> KYSKRIAWMKTTICDSLQLKDMIVEESFQYEKNKNLLEQFLSGEGLNKIFAYYQVQEQAQNDDIKDTGAQDPVLFFTTGDLEKIQDKAVWFLRITNPADDKKKASQQDGNDNDIIFGEITPNTVPMLNALMESVYSRQIDHIITEKIQFWGVAEEEQVLEFQQHSNKFSSEVREAINLMSPGTEHFKLDYEAISGLSESEKMQHYEMKFNEWINLISSQLNDDSEVRKDEKDAGPATELIYWRSRMQKITNWSEQLKSKDFQIVKASLQRHKNHDNQRPRGDESLSKLMMEYNRLDLLLTDKLNEAKDNVKYLTTLEKFIEPLYNGTPQQIIDTLPALMNAIKMIHTIARFYNTTDKMTGLFIKITNQMIKNCKDRILNKKDNGDNPSLYKMIWEQDPAELIEVLGSCIKLYCEYKKCYNDTKEKVADMPKGKTFDFSDAQIFGKFDTFVRRLQKLIEIFSNIQQFNALAKHNLEGMDVLTNKFKKIIDDFKKKGHNLLDTANNKFDRDWVEFNVEISHLDGELQNFIDNNFNRFRNIEYSLKLLHKFQSTIKRDSLKHNLTSRYNAILHNYATELDTIQRVFQDQKSNPPLVRNMPPEAGKIIWARHLFQKITGPINIFPENVINSTEIRRYYGSYNTLGKQLTIYEMWFYQDWVNKIEQSKAALQATLIVRHDENKKLYVNFDLEIMQLIREAKCLDRQGIEIPESARIILLQEDKFKTYYNELLYALKEYERINSKIKPICKNLLLPHIEDLDLKLRPGMVTLTWTSMNIESYLYYVHQGLKKLEQLIINVNDIIENRIENNLKTVSKVVLVHLPQDTKPLSLDSFVQLQEEYINSKTDFLTSKNVEVERAVDDLLQTIMLYPLDPHVDPVLPEETKRIKRYYFWYFYQALLNSTQNSLNAMKYRVCGKKIPGANTLQNLKPFFQVEVQLNGDKVTLNPSLQEIQKSINRAATAVLRCSKHLYNWDQQNKDSTDKATFYDMIACDKEIVKVILLLTGSIQGTKNKVNEFLSGFTKFEWLCKESIQESIKKFSKNGPTLQNYEDQLKKFSQIEEEIEKIVPTYKIGAMELMTHNICTSLSTWAKEWKLQYSQDLHKRARQLLDSLTEQTKMLSTKLSKPVKDIDSLGYVMETLEQIRKEQAEIDMKFNPVQEMYSLLDNYLPGGITDKDEMDARSLLRRNWDILIQQAEIKGKEYQHKQAIYLKELKQSIKDFTNQVSIFRRDYEKNGPMVEGISPAEAMERLRRFEDEYDVKYQMYKINARGENLFGLQNQKYPELEKTDAEIKNLNKLYNLYDSVIKNIQQFKEKSWQDVSKDDLAKMEEDAGKYGEQCSRLPKDLKEWQAYRDLKNYIDSLREQLPLIISLKKPSIMPRHWEKIKEITNTKLNYENPDQFYIEEIMGAKLLDFREDIEDITESADKQLKIRTGLDEINLYWNDMQFQFGIWGKRDVPCMLNGLIVGTILERLEEDQLQLSTFNSQRHVTPFKAEVENLIRTFSDVNDTLDMWVKVQKLWTSLEPVFTGGDIARQMPLQAKQFQGIDKNWMKIMEKAVETKKVIPCCQNDMLKDFLPDLNRKLEDCQKMLEAYLEGKRKKFPRFYFVSNPTLLKILSQGSEPTSIQEDFEKLFDAITKVTFESAKDKKNPALKQITQIQQVIGRNEENISLTGYYVKCEGNIEDWLKKLEQNMQQTLKDIASAAAQQVFQVGLKEFVSSQASQIALLGLQILWTSKVNEGLERLSRNERNAMDIKRNEIKEHMNILSSMCLEDLNGAVERTKVETLVTIQVHQKDISMDLKCKDVNDFEWQKQTRIAWKTDIDECIISITDWDSPYSYEFLGAKERLCITPLTDRCYITLAQAMSMYYGGAPAGPAGTGKTETVKDLGRTLGVFVVVTNCSDQHRYRDMAKIFKGLVQSGLWGCFDEFNRIDLEVLSVVAMQVESITTARKQHMKKFMFPEEEIEIELIPTVSYFITMNPGYAGRQELPENLKVLFRGVSMMVPDREIIIKVKLASVGYLQIDLLAKKFNVLYRLCEEQLSKQRHYDFGLRNILSVLRTAGNTKRQEIKSDEEMLLMRSLRDMNLSKLVADDIPLFNGLLADIFPKLKEVPKKLYPDVEKKIPEEINAESYLINTPSFQLKIIQLYETCLVRHGFMLVGPTGSGKSTIMKILTEVLTKLGSPHKIVIMNPKAITAEQMYGVKSEISDDWIPGVFSTIWAKSNNRALKHTTWITCDGPVDAIWIENLNTVLDDNKILTLANGERIAMTENCKVVFEVENLNNASPATVSRCGQVYVSPTDLGYEAVIEGWIRNRKASGRAEESDKLGNILRKYLINMRFIELQSKECKEPMMDTSPVISVINILNLLTGCLQYFVQTQRTLSEQEYEKFIVYSMAWAIGGIYEAQDRVRFHELLLAKNAPIPQKGKENETVFDYYVSQDYLDWKICSPEEWVPPQSLQFSQLLLPTLDSFRAEMLLNFILTQPKSHTCSNSALLIGGSGTAKTSSVLLYCNKFDPQKMLFKRTNFSSATSPFMFQSTIEAECDFKVGKEFAPPGNKMMTIFIDDMSMPFVNKWGDQITLELVRQLIETGGFYMLDKTQRGNQRKMKNLQYIGAMNHPGGGRNDIPNRLKRQFFIFNMILPLSIEGIYGPIIKHMFKQKYFSDSTYKVIESLTSATIALWNKVKSTMLPTPAKFHYVFNMRELSRIFKGILTCKKDTINDAPKSMKIKPELFLVGLWRHEAERVLADKLVNNKDKDTVMGYIQEVSLESFSQIENEILEKYSSEKTFLFCDFLRPDVINEDGIIEEEAPKIYEAIDSLTELRKRCNFLLSFYNDRNPSKKMPLVLFDDALKHLLRISRIIRQPRSSGLLVGVGGSGKQSLTRLAGFIGKNLIQQIIVTKTYSDKDLKEDIKKGFDDAGHLGKQVTFLMTDSEVKKEEFLEYINMVLSTGEIPNLLAKDEREVWLGDISQAYCKEKNLGNIDPPQSELWTYFVDRVRDNFHIMLCFSPVGQKFRERARKFPALFNECTIDWFLPWPEEALVSVAETFIKNFDKLDTKEETKQELMKHMGNVHLMVNEICDEYYQKMRRQVYVTPKSFLSYLNSYKTLYIEKYDELDQQEESFKIGLNKIQEATITINQMEISLKEEEIQLNEATEKTNQLLANLDKESKKANQKGEEVAATNKQCEIQAEQISKEKEEAERELEAALPALRRAQEAVDSIESKDIVELKANKKPLDIIKYIMNAVLVFFKARLIPIQIEERVFNKKEGKAVLFLKESYDESGIQTLGDMNFMKKLKEFEKDSINEETIELLEPYLNQSEDWFNDTFATKASKAAAGILKWAFAIYEYHQKSKIVKPKRIQVAIAEGRQAIALKELEKAREDLAQIQAYIKNLKDVYTKQMEEKNELEMKAAKTKKKINTARTLITSLSGEKDRWGKGAQDISDQKRKLVGNVSLSTAFISYCGPFNAEYRNKLAQQRFVVDMKKRGVPVTPGLELTSFLIDDATIGEWNLQGLPKDDLSIQNGIMVTNSARYPLFIDPQGQGQNWIRNKLSASIIPERCITTLSHPKFKDMFLKYCMESGLTLIVENIENEVDPMMDPVLERQIIVKGKTQFVNVAGTEMELSKEFKLFMTCRLANPSFSPELSAKTTIIDFTVTQSGLEQQLLGKVISKEQKALEDSLNQLLADVNQNQKDLQRLDKNLLERLINSQGNLLDDTELMDVLNNTKTQAKEVAAKLIDAEIKTKEINEKREQYRPVAIRGSAIYFTMIEVSLVNWMYNSSLEQFLKLFIESIDLSEKAQLPSNRVKNIISFLTFHVYRYVNRGLFEKDKITFILMMAFKILTTAGTISSGDVSLFLKSGDALDIKSERQKQISYLEDNQWLNILALSKHTFSGQTLPFFKELPDLISRSENQWRNWIDKNDPENFPIPDFAESINQEKEIGSFISLCLVRSLRNDRTLIATQNFISNVLGKEFTDPISYPIEGIWQESSNMDPVLFLLSAGADPTSSIDELAKKKKKFPCEKVSMGEGQERVARQVIMKGFVEGGWVILQNCHLGLKFMEEIETLVSPINQIHEDFRLWITCEQHPKFPLGLLQKTLKVTNEPPKGLKAGLYKTFTTIITQEFIDKVDHSNWRSLIFTICFLHSIVIERKKFGPLGWCVPYEYNYSDLEASLLYIEKYLTNLMSTPQPNSHNLPISMNVVRYMICEVQYGGRITDDLDRELFITYGETYLKDGIFGNDYFFY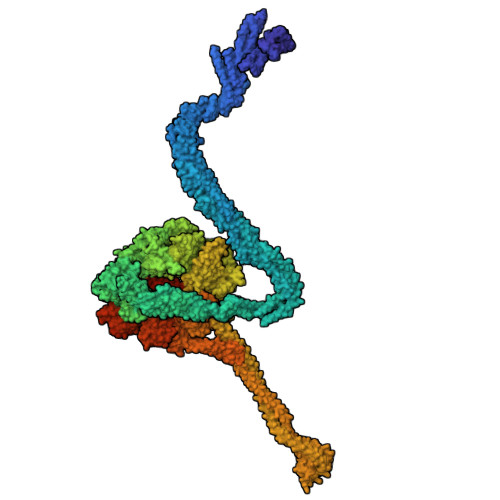DIMVDGSGQKFKYRIPQNPSAELIKYQEYIAKVPTVDNPEVFGLHSNADLTFRLKESKEMINTVMETRPKDSSVGGGKTREEIVQDKAKDMLKNLPPDYNDVEVRELVSKLGGPNPKTSTERGMTVPLNIFLYQEVTRMQRVIGLVRKTLQDTILAIDGQIIMTPEILEAINAIYDAKVPNSWLYDPSGAEISWLLPNLGSWSTSLSDRNKQLNDWLRSGQRPILFWLTGFFNPQGFLTGMKQEVTRNHKKGDGKGGEAWSLDDVVYSTTVKEREKEKDIEQPPAEGVYIKGLYLEGCKWSKNGLDDSDPKKIFADLPILHVSAINKKKTNEQDRMSNTYLCPVYKYPKRTDKYLIFRVGLPCEGSNNPSHWKLRGVALLCST> SITTPEEMIEKAKGETAYLPCKFTLSPEDQGPLDIEWLISPADNQKVDQVIILYSGDKIYDDYYPDLKGRVHFTSNDLKSGDASINVTNLQLSDIGTYQCKVKKAPGVANKKIHLVVL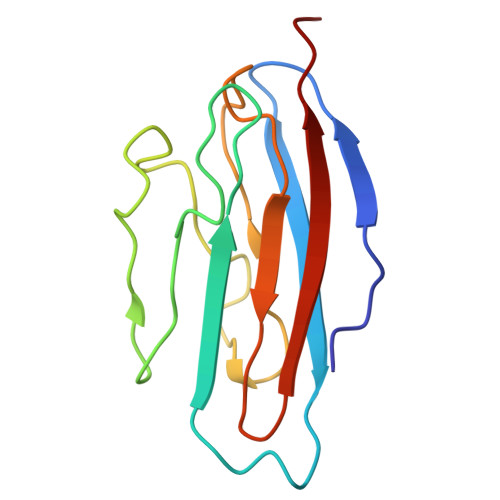VK>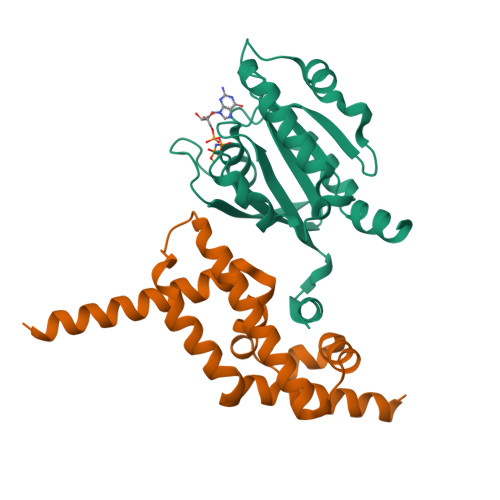[2x]MGLLSILRKLKSAPDQEVRILLLGLDNAGKTTLLKQLASEDISHITPTQGFNIKSVQSQGFKLNVWDIGGQRKIRPYWRSYFENTDILIYVIDSADRKRFEETGQELTELLEEEKLSCVPVLIFANKQDLLTAAPASEIAEGLNLHTIRDRVWQIQSCSALTGEGVQDGMNWVCKNVNAKKKLEHHHHHH;>[2x]GPMAAEEEDEVEWVVESIAGFLRGPDWSIPILDFVEQKCEVFDDEEESKLTYTEIHQEYKELVEKLLESYLKEIGINEDQFQEACTSPLAKTRTSQAILQPVLAAEDFTIFKAMMVQKNIEMQLQAIRIIQERNG>MRLFGYARVSTSQQSLDIQVRALKDAGVKANRIFTDKASGSSSDRKGLDLLRMKVEEGDVILVKK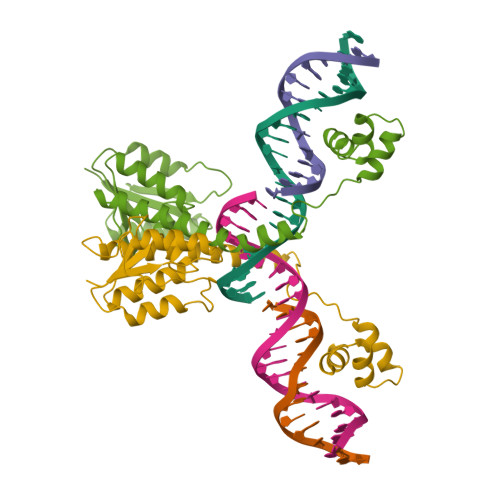LDRLGRDTADMIQLIKEFDAQGVSIRFIDDGISTDGEMGKMVVTILSAVAQAERQRILERTNEGRQEAMAKGVVFGRKRKIDRDAVLNMWQQGLGASHISKTMNIARSTVYKVINESN[2x]> SLLELGKMILQETGKNAITSYGSYGCN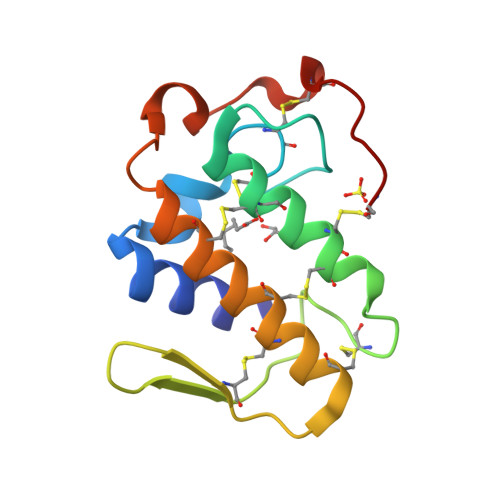CGWGHRGQPKDATDRCCFVHKCCYKKLTDCNHKTDRYSYSWKNKAIICEEKNPCLKEMCECDKAVAICLRENLDTYNKKYKAYFKFKCKKPETC>[3x]MGSSHHHHHSSGENLYFQGHMRSPVQLQHGSDATNGFHTLQPHDQTDGPIKRVCLTRGMHVPEHVAMHHTHDVGPDQCCSSVVQMIHAPPESVWALVRRFDNPKVYKNFIRQCRIVQGDGLHVGDLREVMVVSGLPAVSSTERLEILDEERHVISFSVVGGDHRLKNYRSVTTLHASDDEGTVVVESYIVDVPPGNTEEETLSFVDTIVRCNLQSLARSTNRQ

A 13-member family of ABA receptors PYR/PYL/RCAR (PYLs) in Arabidopsis thaliana was genetically and biochemically identified. Upon binding (+)-ABA, dimeric PYLs underwent a pronounced conformational rearrangement, and then bound and inhibited the group A protein phosphatases type 2Cs (PP2C), including ABI1, ABI2, HAB1 and PP2CA. PYLs/PP2C heterodimer blocked substrates binding to PP2Cs, and thus released downstream transcription factors SnRK2 kinases formerly inhibited by PP2C. Structural analysis along with biochemical data in vitro demonstrated that steric hindrance and hydrophobic interaction in the pocket of PYLs were crucial for their stereospecificity to ABA enantiomers.

PYL5 and PYL9 represent two extremes of recognizing (−)-ABA. PYL5 bound (−)-ABA most strongly, so we first tried to acquire the complex crystal of PYL5 with (−)-ABA. However, the X-ray diffraction data showed that it was highly twinned and could not be merged together. In addition, X-ray diffraction images from apo-PYL5 crystal also showed a highly twin. Nevertheless, the apo-PYL5 structure was solved at a resolution of 2.68 Å. On the contrary, the corresponding two residues in PYL5 and PYL3 were smaller, and thus allowed (−)-ABA to dock into the binding cavity. In addition, the dramatic contrast of binding (−)-ABA between PYL5 and PYL9 also denied the “flip” hypothesis, which supported the hypothesis of dual selectivity of ABA receptor.> MAAAAAAGEARRVLVYGGRGALGSRCVQAFRARNWWVASVDVVENEEASASIIVKMTDSFTEQADQVTAEVGKLLGEEKVDAILCVAGGWAGGNAKSKSLFKNCDLMWKQSIWTSTISSHLATKHLKEGGLLTLAGAKAALDGTPGMIGYGMAKGAVHQLCQSLAGKNSGMPPGAAAIAVLPVTLDTPMNRKSMPEADFSSWTPLEFLVETFHDWI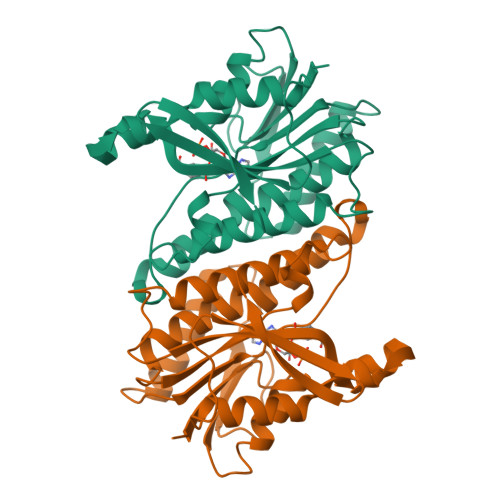TGKNRPSSGSLIQVVTTEGRTELTPAYF> GDVVEAVENAVARVADTIGSGPSNSQAVPALTAVETGHTSQVTPSDTVQTRHVKNYHSRSESSIENFLSRSACVYMGEYHTTNSDQTKLFASWTISARRMVQMRRKLEIFTYVRFDVEVTFVITSKQDQGTQLGQDMPPLTHQIMYIPPGGPIPKSVTDYTWQTSTNPSIFWTEGNAPPRMSIPFISIGNAYSNFYDGWSHFSQNGVYGYNTLNHMGQIYVRHVNGSSPLPMTSTVRMYFKPKHVKAWVPRPPRLCQYKNASTVNFSPTDITDKRNSITYIPDTVKPDVSNH;> SPSAEECGYSDRVRSITLGNSTITTQESANVVVGYGRWPEYLRDDEATAEDQPTQPDVATCRFYTLESVTWEKDSPGWWWKFPDALKDMGLFGQNMYYHYLGRAGYTIHVQCNASKFHQGCLLVVCVPEAEMGCSTVDGTVNEHGLSEGETAKKFSATGTNGTNTVQSI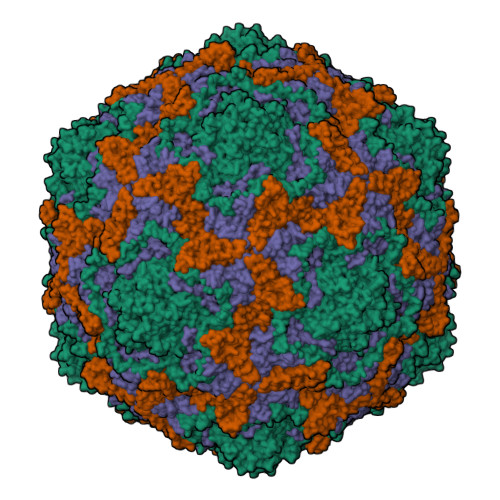VTNAGMGVGVGNLTIFPHQWINLRTNNCATIVMPYINNVPMDNMFRHHNFTLMIIPFVPLNYSSDFSTYVPITVTVAPMCAEYNGLRLSTALQ;> GLPVINTPGSNQFLTSDDFQSPSAMPQFDVTPELNIPGEVQNLMEIAEVDSVVPVNNVAGNLETMDIYRIPVQSGNHQSSQVFGFQVQPGLDGVFKHTLLGEILNYYAHWSGSIKLTFVFCGSAMATGKFLLAYAPPGANAPKSRKDAMLGTHIIWDVGLQSSCVLCIPWISQTHYRLVQQDEYTSAGNVTCWYQTGIVVPAGTPTSCSIMCFVSACNDFSVRLLKDTPFIQQAALLQ;> GAQVSTQKTGAHETGLRASGNSIIHYTNINYYKDAASNSANRQDFTQDPGKFTEPVKDIMVKSLPALN>[2x]MALSLYEKMLHKGMIIKNSNVYEKIKEIDTIIFNKTGTLTYGTPIVTQFIGDSLSLAYAASVEALSSHPIAKAIVKYAKEQGVKILEVKDFKEISGIGVRGKISDKIIEVKKAENNNDIAVYINGEPIASFNISDVP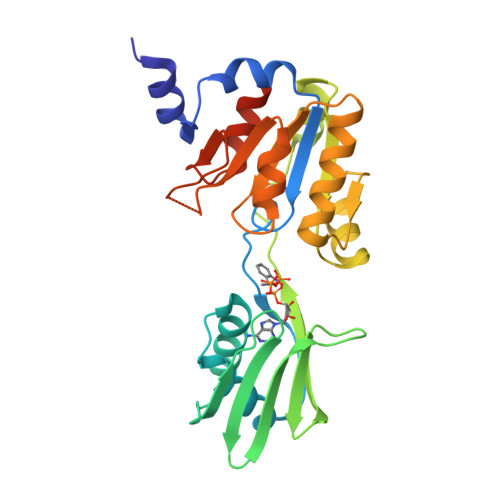RPNLKDYLEKLKNEGLKIIILSGDKEDKVKELSKELNIQEYYSNLSPEDKVRIIEKLKQNGNKVLMIGDGVNDAAALALADVSVAMGNGVDISKNVADIILVSNDIGTLLGLIKNRKRLSNAIPSN>[2x]MGSHHHHHHGRSMSELIKENMHMKLYMEGTVNNHHFKCTSEGEGKPYEGTQTMRIKVVEGGPLPFAFDIL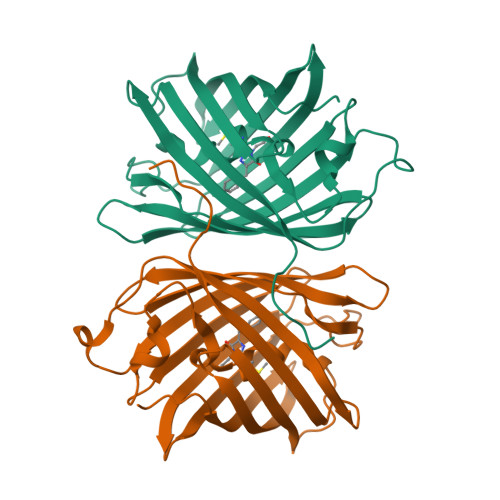ATSFMYGSKTFINHTQGIPDFFKQSFPEGFTWERVTTYEDGGVLTATQDTSLQDGCLIYNVKIRGVNFTSNGPVMQKKTLGWEASTEMLYPADGGLEGRSDEALKLVGGGHLICNLKSTYRSKKPAKNLKVPGVYYVDRRLERIKEADKETYVEQHEVAVARYCDLPSKLGHKLN>[3x]MGSNVNAPRVRRSVRDLQKRYDNGEKKPLEDLVRA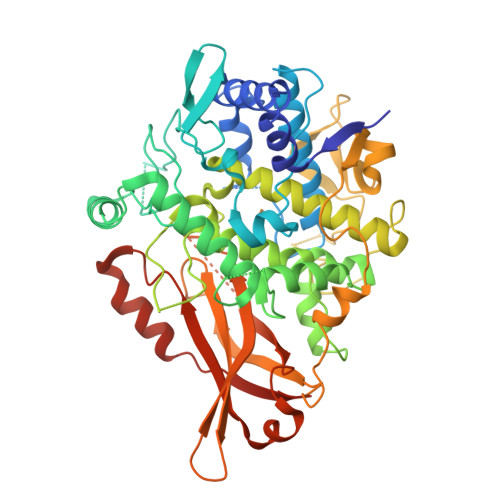WVGIQALPPSDPKSFFALGGYHGEPFQYRKPVDALPQDDIYPYWGGYCNHGNVLFPTWHRMYVYKLEEALQSIVPGVSMPFWDETDEYTLKHGIPSILTQEKFELDGKQIDNPLRSFVLPVALSDRLPGDGNIYEKPKGYVTVRYPLSGLVGTPEALEQTKIHNAKFPLPEKNTELLNSNVRAWLKGDSPTPGDPDPTRNGVYAKYVRCLSAPNYTVFSNTTSASVWNSSNPGLVTPVESPHNDIHLAVGGFDYGGDEIGQIAGANGDMGENNTAGMDPIFFFHHCNVDRMFWVWQKQTGHTDRLDIIRNYPGTNASDSQGPTPGFAPGESLNLTTPLNPFKKASGEAYTSEDCINIERQLGFTYGPGSLDDATPELKSLLAVPSGNSTKKLTVTGIDRAQIQGSFIMKAYASVTDANGKTREYYLGHKSILSRWNVVQCANCLTHLDIVAHFPLSAMPADDVPKAKFRVEFIHRGGGVPSAAKAAIDKVSALQPKFEVSDKLAAALEHHHHHH> MATSGFSKPLHYPPVRRDETVVDDYFGVKVADPYRWLEDPNSEETKEFVDNQEKLANSVLEECELIDKFKQKIIDFVNFPRCGVPFRRANKYFHFYNSGLQAQNVFQMQDDLDGKPEVLYDPNLREGGRSGLSLYSVSEDAKYFAFGIHSGLTEWVTIKILKTEDRSYLPDTLEWVKFSPAIWTHDNKGFFYCPYPPLKEGEDHMTRSAVNQEARYHFLGTDQSEDILLWRDLENPAHHLKCQITDDGKYFLLYILDGCDDANKVYCLDLTKLPNGLESFRGREDSAPFMKLIDSFDASYTAIANDGSVFTFQTNKDAPRKKLVRVDLNNPSVWTDLVPESKKDLLESAHAVNENQLILRYLSDVKHVLEIRDLESGALQHRLPIDIGSVDGITARRRDSVVFFKFTSILTPGIVYQCDLKNDPTQLKIFRESVVPDFDRSEFEVKQVFVPSKDGTKIPIFIAARKGISLDGSHPCEMHGYGGFGINMMPTFSASRIVFLKHLGGVFCLANIR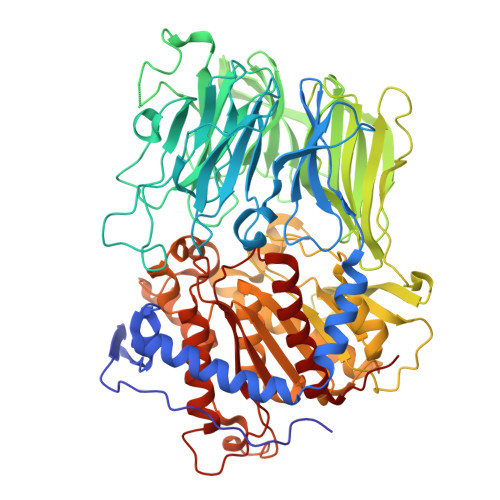GGGEYGEEWHKAGFRDKKQNVFDDFISAAEYLISSGYTKARRVAIEGGANGGLLVAACINQRPDLFGCAEANCGVMDMLRFHKFTLGYLWTGDYGCSDKEEEFKWLIKYSPIHNVRRPWEQPGNEETQYPATMILTADHDDRVVPLHSFKLLATMQHVLCTSLEDSPQKNPIIARIQRKAAHYGRATMTQIAEVADRYGFMAKALEAPWID~{N}-[(5-azanyl-1,3,4-oxadiazol-2-yl)methyl]-2-(2-chlorophenyl)sulfanyl-~{N}-[(6-oxidanylidene-1~{H}-pyridin-3-yl)methyl]ethanamide | C17 H16 Cl N5 O3 S | 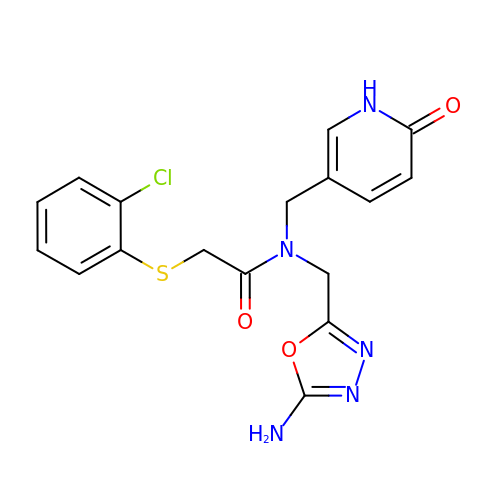YRQRMFRLHMFRAP-UHFFFAOYSA-N> MASETPRVDPTEISNVNAPVFRIIAQIKSQPTESQLILQSPTISSKNGSEVEMITLNNIRVSMNKTFEIDSWYEFVCRNNDDGELGFLILDA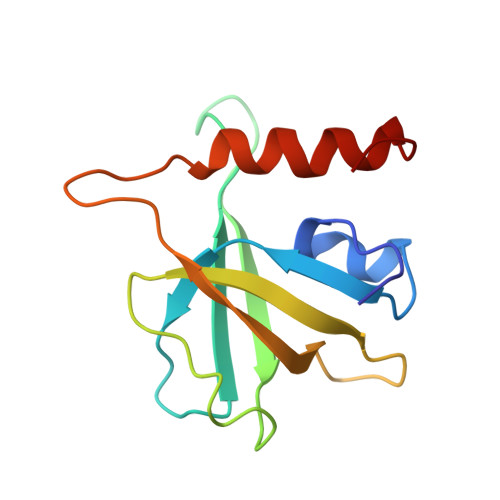VLCKFKENEDLSLNGVVALQRLCKKYPEIY>[4x]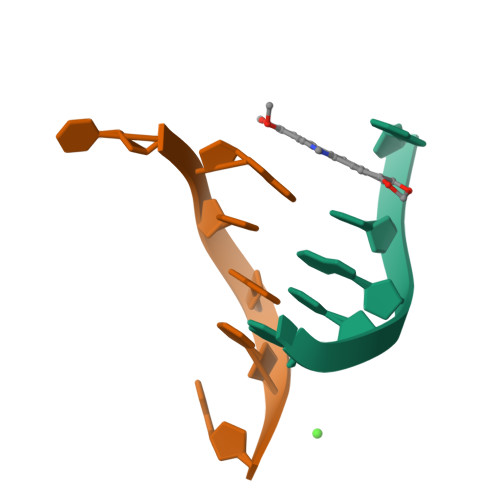CGTACG>MNNTIINSLIGGDDSIKRSNVFAVDSQIPTLYMPQYISLSGVMTNDGPDNQAIASFEIRDQYITALNHLVLSLELPEVKGMGRFGYVPYVGYKCINHVSISSCNGVIWEIEGEELYNNCINNTIALKHSGYSSELNDISIGLTPNDTIKEPSTVYVYIKTPFDVEDTFSSLKLSDSKITVTVTFNPVSDIVIRDSSFDFETFNKEFVYVPELSFIGYMVKNVQIKPSFIEKPRRVIGQINQPTATVTEVHAATSLSVYTKPYYGNTDNKFISYPGYSQDEKDYIDAYVSRLLDDLVIVSDGPPTGYPESAEIVEVPEDGIVSIQDADVYVKIDNVPDNMSVYLHTNLLMFGTRKNSFIYNISKKFSAITGTYSDATKRTIFAHISHSINIIDTSIPVSLWTSQRNVYNGDNRSAESKAKDLFINDPFIKGIDFKNKTDIISRLEVRFGNDVLYSENGPISRIYNELLTKSNNGTRTLTFNFTPKIFFRPTTITANVSRGKDKLSVRVVYSTMDVNHPIYYVQKQLVVVCNDLYKVSYDQGVSITKIMGDNN[6x]

During its cytoplasmic replication, vaccinia virus assembles non-infectious spherical immature virions (IV) coated by a viral D13 lattice. The characteristic dimensions and shape of the crescents are determined and maintained by the D13 scaffolding viral protein, which forms trimers that assemble into a hexameric lattice coating the outer surface of these membranes. In vitro structural analysis of recombinant D13 reveals it has a double-jelly-roll structure composed of 8 antiparallel β-strands that self assembles into a honeycomb lattice of pseudohexagonal trimers. During this maturation process, the D13 honeycomb lattice is lost, and a biconcave viral core, containing the viral genome, assembles inside the IV.

Given the clear lattices present on the IV surface in our tomograms, we analysed the structure of the D13 lattice in situ by STA. We obtained maps by averaging surface sectors revealing hexamers of trimer arrangements with a lattice spacing of 133 Å, in agreement with lattices described for in vitro assembled D13 and deep-etch EM honeycombs. We found that the D13 lattices coating IV have a similar architecture to the D13 lattices formed in vitro. From the hexagonal packing of D13 in the subtomogram average, we estimate that approximately 5,300 D13 trimers will cover the surface of a spherical IV. The packing density and radius of the D13 lattice on IV are compatible with an icosahedrally symmetric architecture with a triangulation number (T) in the neighbourhood of 268. We have not confirmed the presence of icosahedral symmetry, which would require pentameric arrangements of D13 trimers, such as those that have been identified in vitro. Finally, we observed a gap of approximately 5.6 nm between the innermost surface of the D13 lattice and the membrane of the IV. This gap cannot be explained by any unresolved N- or C-terminal residues of D13 and must therefore be bridged by another protein such as A17. Analysis of tomograms in 3D, however, reveals that a proportion of IV despite being closed and fully coated by D13 have a single invagination of the viral membrane. This suggests that the D13 lattice is flexible and can accommodate both positive and negative curvatures present on virions with invaginations. Furthermore, Hyun and colleagues produced D13 spherical IV-like particles with a similar diameter to the D13-coated IV we imaged in situ. This strongly suggests that the D13 lattice, which initially curves open membranes and eventually forms closed particles, determines both the size and shape of the IV.2-[2-[[3-[3-(aminomethyl)phenyl]phenyl]carbonylamino]phenyl]ethanoic 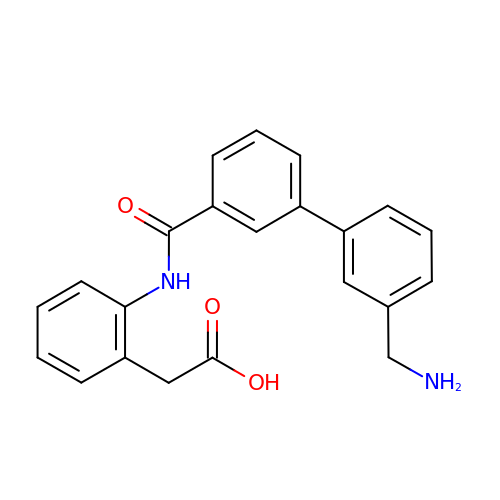acid | C22 H20 N2 O3 | VEQODTWEXCBUAZ-UHFFFAOYSA-N(2S,3S)-4-cyclopropyl-3-{(3R,5R)-3-[2-fluoro-4-(methylsulfonyl)phenyl]-1,2,4-oxadiazolidin-5-yl}-1-[(3S)-3-fluoropyrrolidin-1-yl]-1-oxobutan-2-amine | C20 H28 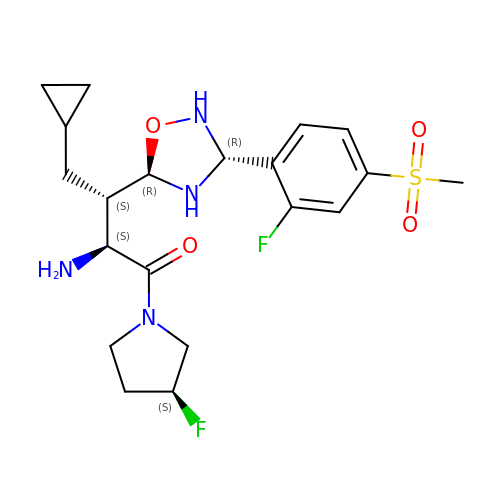F2 N4 O4 S | PTAHVQJZNFGPHN-WFWWEWPISA-N> NIKETLQKIKEVVLEIMDKGDDEQIKLAQSLLIVAEIAVAVGDKETVEKMYKEAKYILDNINSITDEEIKKMLEEAAKIAKKLLEKAKDLPEEERILLRIKALVIEVMAYGDDETIKEAQKLLIKAELAVKEGDLETLKKILKE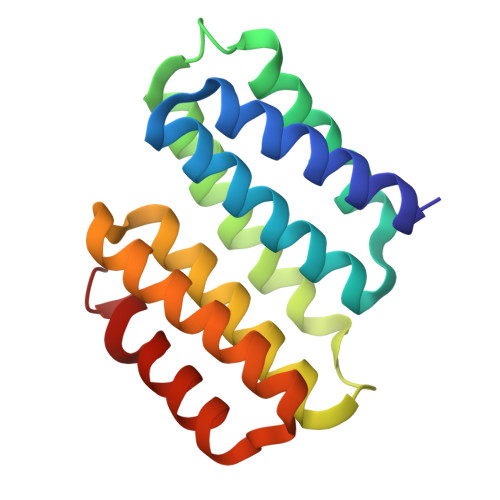MEKMVKEVK DIETHYL PROPANE-1,3-DIYLBISCARBAMATE 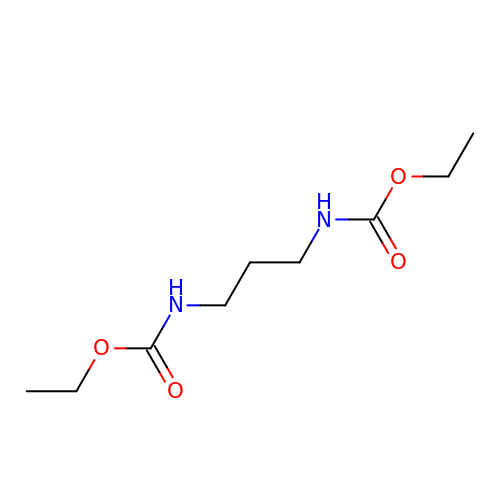| C9 H18 N2 O4 | BWWHOVJFNMPUKF-UHFFFAOYSA-N> GSPSKTKSAPVSYDKDGMNASEEDFSFDNTLAKPYEPLYARRGDI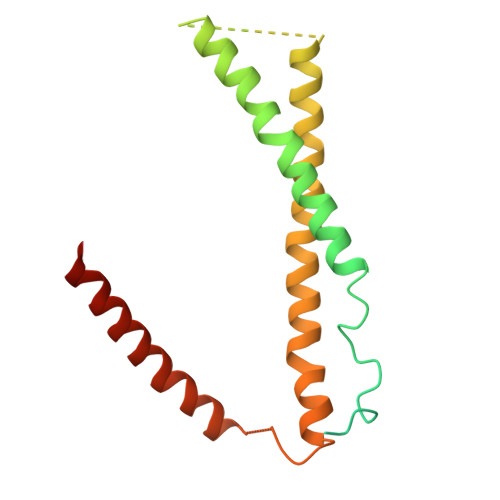TSAGSTSGEDSSQPKMITISGEQLNLITENKELMNELTLVSTELAESIKRETELEERIRLYETNNSAPSFDDSSSVSFSDFEKELRKKSSKIVQLIQQLNDERLKRFIAEEQLLLQENGTKPSSMELVGRIENLNKLIDERDSEIEMLKGRLQ> MSSPVIGITFGNTSSSIAYINPKNDVDVIANPDGERAIPSALSYVGEDEYHGGQALQQLIRNPKNTIINFRDFIGLPFDKCDVSKCANGAPAVEVDGKVGFVISRGEGKEEKLTVDEVVSRHLNRLKLAAEDYIGSAVKEAVLTVPTNFSEEQKTALKASAAKIGLQIVQFINEPSAALLAHAEQFPFEKDVNVVVADFGGIRSDAAVIAVRNGIFTILATAHDLSLGGDNLDTELVEYFASEFQKKYQANPRKNARSLAKLKANSSITKKTLSNATSATISIDSLADGFDYHASINRMRYELVANKVFAQFSSFVDSVIAKAELDPLDIDAVLLTGGVSFTPKLTTNLEYTLPESVEILGPQNKNASNNPNELAASGAALQARLISDYDADELAEALQPVIVNTPHLKKPIGLIGAKGEFHPVLLAETSFPVQKKLTLKQAK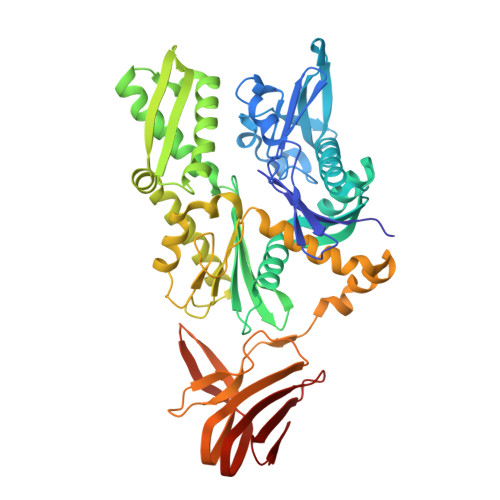GDFLIGVYEGDHHIEEKTLEPIPKEENAEEDDESEWSDDEPEVVREKLYTLGTKLMELGIKNANGVEIIFNINKDGALRVTARDLKTGNAVKGEL>[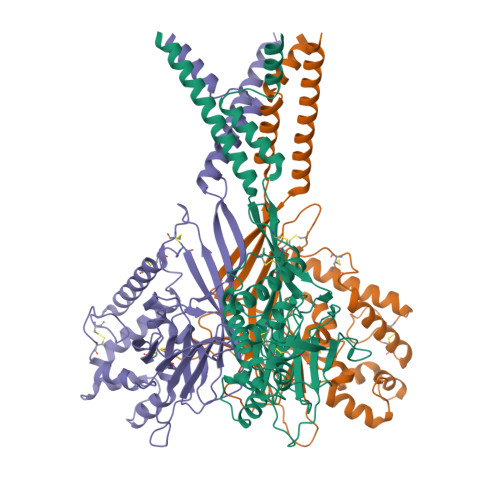3x]MAPSAYALDRSSVPSGKPRLMEGAESKARAGARKIHHLKIHGFDRVFGPGTHRWQRALWFAGVVFCFGISAHQIAMHVLDYLSEPVAVRIDFVAQNELRIPEITVCPRIFQQNTIFTDMVEKQGIDKMKFLDLIDRPEYDIMAVWNLSRIFSDNVSCSAHEGSSIISGSYVDPNMSQPHLVYTTSGQCINIPASRPLIYRGVNTFVRITDSQPRNLDEVRPEAIQIYFHEHHHAHLSRYLTGLRGYIVPIANPFAFSIRFTQINYANRTDSPCVDSEEYAACVEDFIEQRIYEKAQVQCRLPYMRPKLPLCSTPTDARKIFVATDDVIQNFEKESSCKRKCEENLYIVEFMHLFERSNISIDMSVYFAYNYIQVATEYLTYTLRGLLSDIGGVLGLFLGICILSVIEVFEVVIFSLQRVLCNEDKKQQNNE>GHMKVK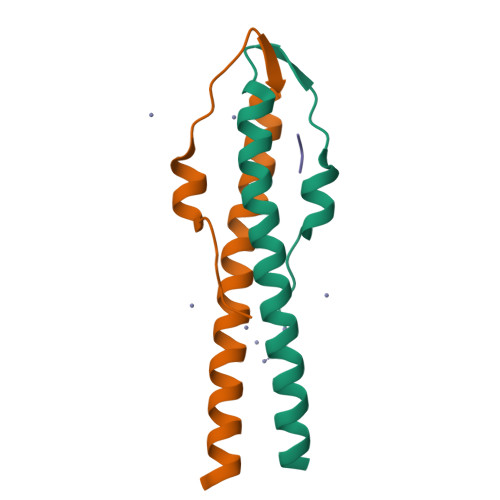LSAKEILEKEFKTGVRGYKQEDVDEFLDMIIKDYETFHQEIEELQQENLQLKKQLEE[2x];> MADKPQTRSQYRNKQ> STMAIEKILTDAKTLLERLREHDAAAESLVDQSAALHRRVAA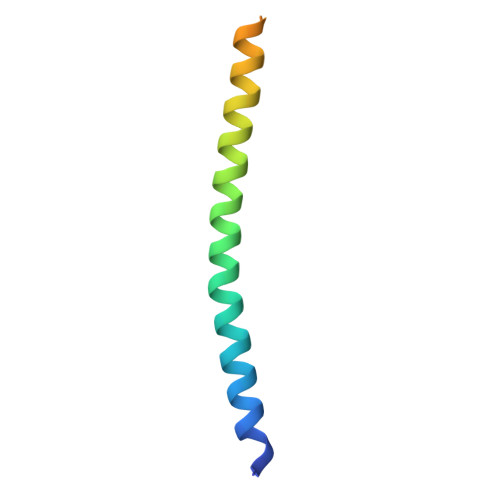MREAGTALPDQYQEDASDMKDMS>GSHMGHWSQGLKISMQDPKMQVYKDEQVVVIKDKYPKARYQWLVLPWTSISSLKAVAREHLELLKHMHTVGEKVIVDFAGSSKLRFRLGYHAIPSMSHVHLHVISQDFDSPCLKNKKHWNSFNTEYFLESQAVIEMVQEAGRVTVRDGMPELLKLPLRCHECQQLLPSIPQLKEHLRKHW[2x]

The APTX RNA‐DNA deadenylase protects genome integrity and corrects abortive DNA ligation arising during ribonucleotide excision repair and base excision DNA repair, and APTX human mutations cause the neurodegenerative disorder ataxia with oculomotor ataxia 1 (AOA1). The aprataxin (APTX) RNA/DNA polynucleotide deadenylase directly reverses 5′‐AMP damage (Ahel et al, 2006; Harris et al, 2009; Reynolds et al, 2009; Tumbale et al, 2011, 2014) and associates with DNA repair scaffolds XRCC1 (Cherry et al, 2015) and XRCC4. Environmental and metabolic sources of DNA damage prompt “abortive ligation”, the failure of ligase to complete step 3, and generation of 5′‐adenylated (5′‐AMP) DNA strand breaks (Ahel et al, 2006; Andres et al, 2015; Schellenberg et al, 2015). AOA1 mutations map to the APTX catalytic domain (Barbot et al, 2001; Moreira et al, 2001; Shimazaki et al, 2002; Le Ber et al, 2003; Tranchant et al, 2003; Criscuolo et al, 2004, 2005; Ito et al, 2005; Mosesso et al, 2005; Baba et al, 2007; Yokoseki et al, 2011) and cause variable age of disease onset.

H201Q: While His201 falls outside of the so‐called HIT domain histidine triad motif, it is highly conserved in HIT domain phosphohydrolases, including APTX homologs. Based on the structure of an adenosine‐vanadate transition‐like state mimic, it is proposed that His201 enables stabilization of the negatively charged transition state of the deadenylation reaction (Tumbale et al, 2014; Schellenberg et al, 2015) via its participation in a charge relay consisting of the main‐chain backbone of Lys197, His201, and His262 that hydrogen bonds to the scissile phosphate of the 5′‐AMP phosphoanhydride. The high‐resolution structure of H201Q (at 1.65 Å) reveals the effects of this substitution on active site chemistry from the histidine to glutamine mutation. In the structure of the H201Q mutant, although the active site undergoes minimal gross structural rearrangements, this charge relay is compromised, likely resulting in the significant reduction in catalytic activity and protein stability. Intriguingly, while seemingly well accommodated in the active site, the H201Q substitution also confers substantial temperature‐dependent effects on catalysis. Close analysis of the backbone conformations of the Tyr200‐Gln201 peptide bond reveals that a strained, but permissible deviation of peptide bond planarity (172–173°) is observed compared to wild‐type APTX (Tumbale et al, 2014). This non‐native backbone conformation in part could explain the thermal stability defect for H201Q. Precisely how the H201Q substitution disrupts the APTX charge relay system will require future NMR or neutron scattering analysis of active site protonation states.>[2x]MSSSHHHHHHMPTKKQKSKSKLKPFFALV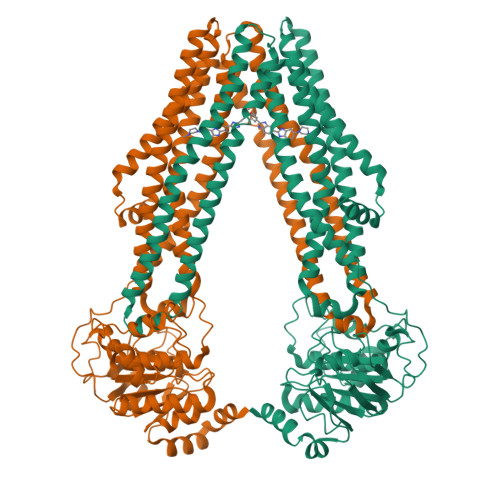RRTNPSYGKLAFALALSVVTTLVSLLIPLLTKQLVDGFSMSNLSGTQIGLIALVFFVQAGLSAYATYALNYNGQKIISGLRELLWKKLIKLPVSYFDTNASGETVSRVTNDTMVVKELITTHISGFITGIISVIGSLTILFIMNWKLTLLVLVVVPLAALILVPIGRKMFSISRETQDETARFTGLLNQILPEIRLVKASNAEDVEYGRGKMGISSLFKLGVREAKVQSLVGPLISLVLMAALVAVIGYGGMQVSSGELTAGALVAFILYLFQIIMPMGQITTFFTQLQKSIGATERMIEILAEEEEDTVTGKQIENAHLPIQLDRVSFGYKPDQLILKEVSAVIEAGKVTAIVGPSGGGKTTLFKLLERFYSPTAGTIRLGDEPVDTYSLESWREHIGYVSQESPLMSGTIRENICYGLERDVTDAEIEKAAEMAYALNFIKELPNQFDTEVGERGIMLSGGQRQRIAIARALLRNPSILMLDAATSSLDSQSEKSVQQALEVLMEGRTTIVIAHRLSTVVDADQLLFVEKGEITGRGTHHELMASHGLYRDFAEQQLKMNADLENKAG(2E)-2-[({3-HYDROXY-2-METHYL-5-[(PHOSPHONOOXY)METHYL]PYRIDIN-4-YL}METHYL)AMINO]-5-PHOSPHONOPENT-2-ENOIC ACID | C13 H20 N2 O10 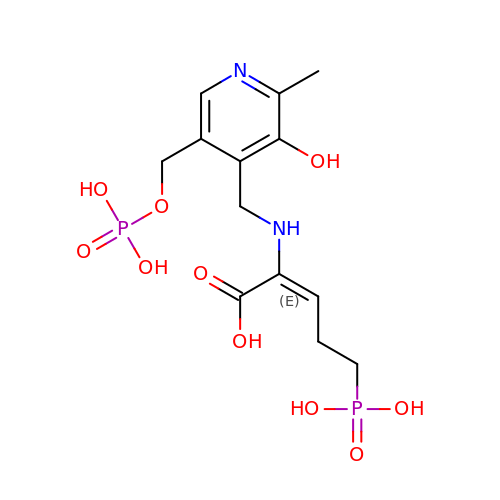P2 | TVSPSLFYIKMGSC-QDEBKDIKSA-N PYROGLUTAMIC ACID | C5 H7 N 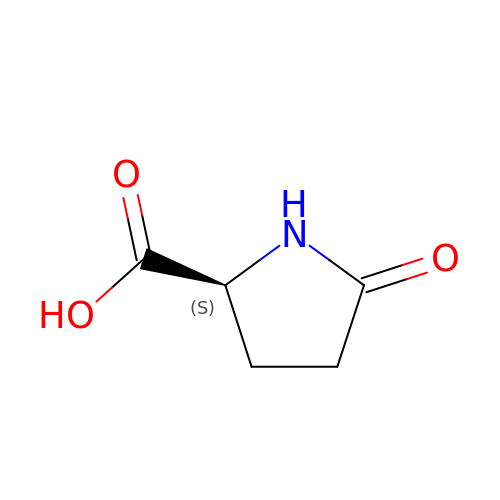O3 | ODHCTXKNWHHXJC-VKHMYHEASA-N>[6x]GAMAKVQVNNVVVLDNPSPFYNPFQFEITFECIEDLSEDLEWKIIYVGSA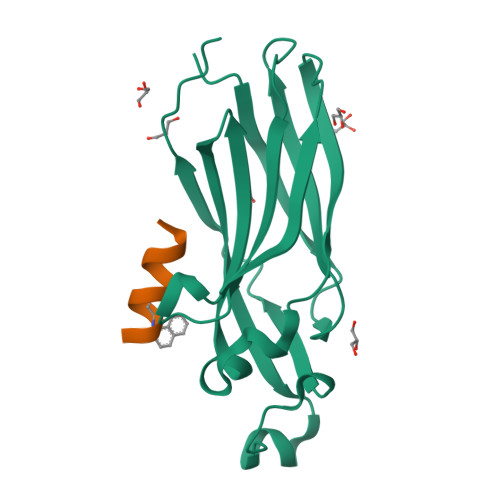ESEEYDQVLDSVLVGPVPAGRHMFVFQADAPNPGLIPDADAVGVTVVLITCTYRGQEFIRVGYYVNNEYTETELRENPPVKPDFSKLQRNILASNPRVTRFHINWEDN;>XEKAARLARRIAX[6x]>[2x]MKSALSDLAFFGGPAAFDQPLLVGRPNRIDRARLYERLDRALDSQWLSNGGPLVREFEERVAGLAGVRHAVATCNATAGLQLLAHAAGLTGEVIMPSMTFAATPHALRWIGLTPVFADIDPDTGNLDPDQVAAAVTPRTSAVVGVHLWGR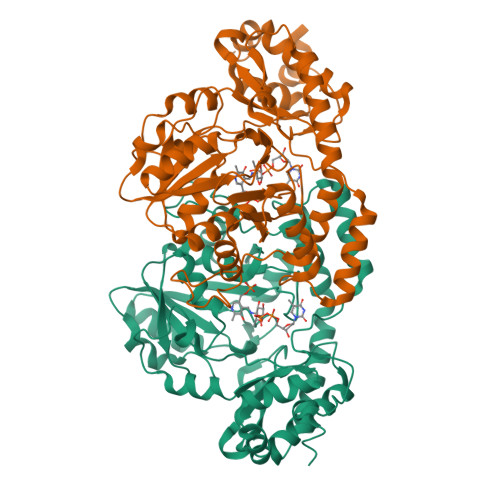PCAADQLRKVADEHGLRLYFDAAHALGCAVDGRPAGSLGDAEVFSFHATKAVNAFEGGAVVTDDADLAARIRALHNFGFDLPGGSPAGGTNAKMSEAAAAMGLTSLDAFPEVIDRNRRNHAAYREHLADLPGVLVADHDRHGLNNHQYVIVEIDEATTGIHRDLVMEVLKAEGVHTRAYFSPGCHELEPYRGQPHAPLPHTERLAARVLSLPTGTAIGDDDIRRVADLLRLCATRGRELTARHRDTAPAPLAAPQTSTPTIGRSRGLEHHHHHH> ETGKIFCKSVSKDPDFRLKQIDYVIPVQQDRSICMNNPLLDISDGFFTYIHYEGINSCKKSDSFKVLLSHGEIVDRGDYRPSLYLLSSHYHPYSMQVINCVPVTCNQSSFVFCHISNNTKTLDNSDYSSDEYYITYFNGIDRPKTKKIPINNMTADNRYIHFTFSGGGGVCLGEEFIIPVTTVINTDVFTHDYCESFNCSVQTGKSLKEICSESLRSPTNSSRYNLNGIMIISQNNMTDFKIQLNGITYNKLSFGSPGRLSKTLGQVLYYQSSMSWDTYLKAGFVEKWKPF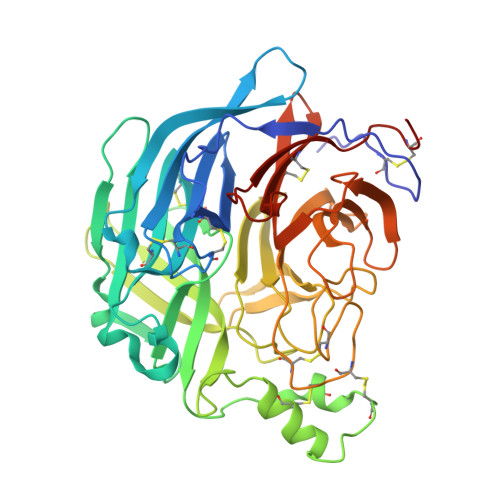TPNWMNNTVISRPNQGNCPRYHKCPEICYGGTYNDIAPLDLGKDMYVSVILDSDQLAENPEITVFNSTTILYKERVSKDELNTRSTTTSCFLFLDEPWCISVLETNRFNGKSIRPEIYSYKIPKYCGTKHHHHHH>[2x]GAMGSGIQRPTSTSSLVAAMATRGANVIWFRHGLRLHDNPALLAALADKDQGIALIPVFIFDGESAGTKNVGYNRMRFLLDSLQDIDDQLQAATDGRGRLLVFEGEPAYIFRRLHEQVRLHRICIEQDCEPIWNERDESIRSLCRELNIDFVEKVSHTLWDPQLV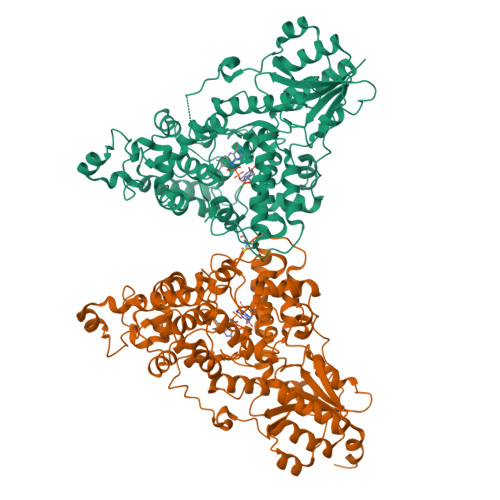IETNGGIPPLTYQMFLHTVQIIGLPPRPTADARLEDATFVELDPEFCRSLKLFEQLPTPEHFNVYGDNMGFLAKINWRGGETQALLLLDERLKVEQHAFERGFYLPNQALPNIHDSPKSMSAHLRFGCLSVRRFYWSVHDLFKNVQLRACVRGVQMTGGAHITGQLIWREYFYTMSVNNPNYDRMEGNDICLSIPWAKPNENLLQSWRLGQTGFPLIDGAMRQLLAEGWLHHTLRNTVATFLTRGGLWQSWEHGLQHFLKYLLDADWSVCAGNWMWVSSSAFERLLDSSLVTCPVALAKRLDPDGTYIKQYVPELMNVPKEFVHEPWRMSAEQQEQYECLIGVHYPERIIDLSMAVKRNMLAMKSLRNSLITPPPHCRPSNEEEVRQFFWLADVVV>MSDSSPTINFINFNQTGTCISLGTSKGFKIFNCEPFGKFYSEDSGGYAIVEMLFSTSLLALVGIGDQPALSPRRLRIINTKKHSIICEVTFPTSILSVKMNKSRLVVLLQEQIYIYDINTMRLLHTIETNPNPRGLMAMSPSVANSYLVYPSPPKVINSEIKAHATTNNITLSVGGNTETSFKRDQQDAGHSDISDLDQYSSFTKRDDADPTSSNGGNSSIIKNGDVIVFNLETLQPTMVIEAHKGEIAAMAISFDGTLMATASDKGTIIRVFDIETGDKIYQFRRGTYATRIYSISFSEDSQYLAVTGSSKTVHIFKLGHSMSNNKLDSDDSNMEEAAADDSSLDTTSIDALSDEENPTRLAREPYVDASRKTMGRMIRYSSQKLSRRAARTLGQIFPIKVTSLLESSRHFASLKLPVETNSHVMTISSIGSPIDIDTSEYPELFETGNSASTESYHEPVMKMVPIRVVSSDGYLYNFVMDPERGGDCLILSQYSILMD[4x]

Autophagy-related protein 18 (Atg18) participates in the elongation of early autophagosomal structures in concert with Atg2 and Atg9 complexes. Atg18 belongs to the protein family of β-propellers that bind polyphosphoinositides (PROPPIN). The corresponding primary structure contains a series of conserved WD40 repeats forming the 6 or 7 blades of a β-propeller fold. The autophagic membrane adapter Atg18 reveals an unexpected structural plasticity in multiple modes of oligomeric organization.

Interestingly, once dialyzed into the low-salt buffer (100 mM KCl), Atg18 formed large supramolecular structures when imaged in negatively stained EM samples. Using cryo-EM of vitrified Atg18, we identified helical tubes of 260 Å diameter including a diamond-shape repeat pattern along the helix. We acquired cryo-EM micrographs of wildtype Atg18 (Atg18-WT) and subjected them to segmented helical image processing. 2D class averages of the helical tubes revealed individual Atg18 propeller disc-shaped structures including individual blade separation. The assemblies exhibited a pitch of ~100 Å with 5.1 helical units per turn. D Fourier shell correlation threshold at 0.143 indicates resolutions of 3.8 and 3.3 Å for the 3D structures of Atg18-WT and Atg18-PR72AA, respectively. The determined cryo-EM structures of Atg18-WT and Atg18-PR72AA constitute two main propeller interactions mediated by the T and I-interface between neighboring monomers. Interestingly, the lipid binding sites appear buried in the T-interface of the helical tube suggesting a stabilizing role of the involved residues. In line with the highest affinity, we found that PI3,5P2 binding leads to disassembly of the helical tubes.> XMNFSGKYQVQSQENFEPFMKAMGLPEDLIQKGKDIKGVSEIVHEGKKVKLTITYGSKVIHNEFTLGEECELETMTGEKVKAVVKMEGDNK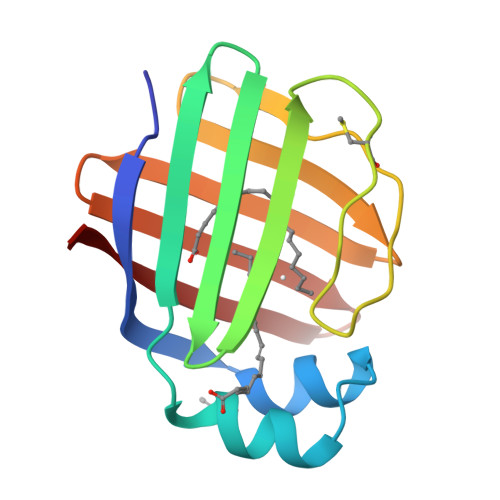MVTTFKGIKSVTEFNGDTITNTMTLGDIVYKRVSKRI> MHHHHHHLVPRGSPSPPGNLRVTDVTSTSVTLSWEPPPGPITGYRVEYREAGGEWKEVTVPGSETSYTVTGLKPGTEYEFRVRAVNGAGEGPPSSVSVTT

We selected the fibronectin type III (FN3) domain, a small β-sheet sandwich of roughly 90–100 amino acids in length, due to its ubiquitous nature across phyla, and its popularity as a model for protein folding and engineering studies. This paper describes the structural and biophysical characterization of FN3con—a consensus-derived FN3 domain having increased stability. We generated the new protein sequence using the consensus method, which selects the most frequently observed residue at each column of the sequence alignment. Design of FN3con was carried out by complete sequence generation using 2123 homologous FN3 domain sequences.

In order to understand the structural basis for stability in FN3con, we determined its X-ray crystal structure to 2.0 Å resolution. FN3con adopts the FN3 fold, consisting of seven anti-parallel β-strands connected by surface exposed loops. A structural alignment with our comparison domains shows very high similarity, with an average root mean square deviation (RMSD) of 1.2 Å across backbone Cα atoms in all structures. Analysis reveals FN3con to have the highest number of H-bonds and salt bridges, with the smallest accessible surface area (ASA). Interestingly, FN3con harbors a unique and extensive complementary charged electrostatic network that is distributed over β-sheet 2, spanning strands C′, C and F. This network results from the presence of four arginine residues and four glutamic acid residues (R45, R49, R81, R83, and E47, E57, E79, E90), which are not present in any of the other FN3 domains. The most striking observation from these calculations is the significantly reduced solvent inaccessible cavity volume of FN3con (60.8 Å3) compared with the next most stable domain, Fibcon (171.0 Å3). All assessed FN3 domains contain the highly conserved tryptophan 22 (W22), while FN3con further contains a unique solvent-exposed tryptophan (W55) on β-sheet 2. W55 packs tightly against the side chains of E47, R49, E79 and R81; however, its effect on stability is not immediately apparent. The hydrophobic core of FN3con is highly regular, exhibiting uniform banding of hydrophobic residues. Structural analysis of FN3con revealed the introduction of a cooperative electrostatic network, optimization of the hydrophobic core packing and accumulation of tyrosine corner residues in a positional pattern that is not seen in any of the other FN3 domains assessed.>[2x]A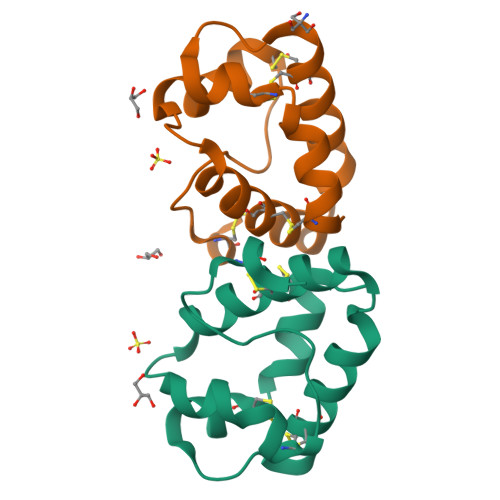VTCGQVDANLAPCVPFLTQGGEPGAACCSGVKTLNGNAQSPDDRKTACNCIKAAANRYPNLKDDAAQSLPSKCGISLNVPISRTINCDTIS> MHHHHHHSSGRENLYFQGDLQATPGMFITSKKGHLSEMYQRVKKLGSGAYGEVLLCRDKVTHVERAIKIIRKTSVSTSSNSKLLEEVAVLKLLDHPNIMKLYDFFEDKRNYYLVMECYKGGELF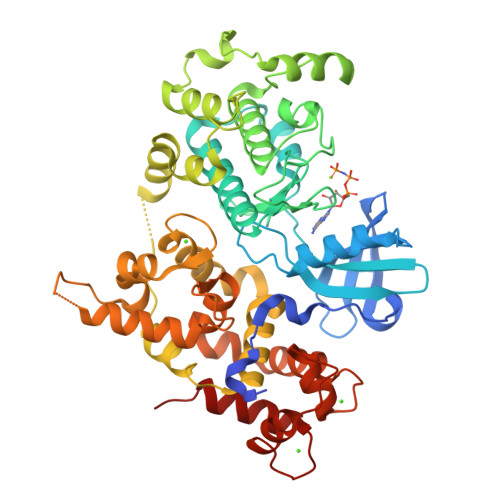DEIIHRMKFNEVDAAVIIKQVLSGVTYLHKHNIVHRDLKPENLLLESKEKDALIKIVDFGLSAVFENQKKMKERLGTAYYIAPEVLRKKYDEKCDVWSIGVILFILLAGYPPFGGQTDQEILRKVEKGKYTFDSPEWKNVSEGAKDLIKQMLQFDSQRRISAQQALEHPWIKEMCSKKESGIELPSLANAIENMRKFQNSQKLAQAALLYMASKLTSQEETKELTDIFRHIDKNGDGQLDRQELIDGYSKLSGEEVAVFDLPQIESEVDAILGAADFDRNGYIDYSEFVTVAMDRKSLLSKDKLESAFQKFDQDGNGKISVDELASVFGLDHLESKTWKEMISGIDSNNDGDVDFEEFCKMIQKLCSNNE>[2x]MIELSLAEALFLILFTGVISMLISRRTGISYVPIFILTGLVIGPLLKLIPRDLAHEIFDFVRVFGLVIILFTEGHNLSWRLLKKNMPTIVTLDTIGLILTALIAGFIFKVVFNSSFLLGFLFGAIIGATDPATLIPLFRQYRVKQDIETVIVTESIFNDPLGIVLTLIAISMLVPGYGGGIFSTLSEKLGIYAGGVIYFLYNVSVSISLGIFLGILGYKFIKRTGIFDFPEIEAFSLSLAFLGFFIGERLDASGYLVATVTGIVLGNYKLLKPRENIRILKRLQRAIEKEVHFNDTLAALATIFIFVLLGAEMNLEVIWSNLGKGLLVALGVMILARPLATLPLLKWWNFREYLFIALEGPRGVVPSALASLPLSLALKYKSPLLTVHWGEIIMATVVITVLTSVIVETLWIPILKDKLDVG

H5 and H12 in the 6-helix bundle are discontinuous. dimer indicates clusters of charged residues on both sides of the membrane. transported by PaNhaP, K+ is not. structure thus serves as an excellent model for the membrane part of NHE1.

The structure of PaNhaP crystals grown at pH 4 was determined at 3.5 Å by molecular replacement. conspicuous differences to the pH 8 structure are observed near the dimer interface. Six ion bridges that lock the two protomers together at pH 8 break at pH 4. As a result, the two protomers tilt away from each other at lower pH. the cytoplasmic end of H1 and H7/8 present at pH 8 break at pH 4. the 6-helix bundle, but significant rearrangements at the dimer interface. site in protomer B changes only slightly from pH 8 to pH 4.Bacillus phages use a communication system, termed “arbitrium,” to coordinate lysis-lysogeny decisions. Arbitrium communication is mediated by the production and secretion of a hexapeptide (AimP) during lytic cycle. Once internalized, AimP reduces the expression of the negative regulator of lysogeny, AimX, by binding to the transcription factor, AimR, promoting lysogeny. We have elucidated the crystal structures of AimR from the Bacillus subtilis SPbeta phage in its apo form, bound to its DNA operator and in complex with AimP.

To establish the molecular basis of this novel mechanism of phage communication we produced crystals of AimR in its apo form that diffracted to 2.7Å and belong to space group P21 with eight monomers in the asymmetric unit. The overall structure of each monomer shows an N-terminal HTH DNA-binding domain (residues 1–59) directly connected (only 2 residues) to a C-terminal regulatory domain (residues 62–386) composed of 18 helices arranged in a two-layered right-handed superhelix. The HTH motif includes 4 helices (helix α1–α4), and the predicted DNA recognition helix α3 is solvent exposed, which is compatible with the active DNA-binding state proposed for the apo protein (Erez et al., 2017). Sequence analysis with TPRpred server (Zimmermann et al., 2018) only predicts the presence of four TPR, but the structure showed that the 18 α helices of C-terminal domain could be organized in 9 TPR-like motifs if helix α4 of the HTH domain was part of the first TPR. These 9 TPR-like motifs (TPR1–9), unlike other members of the RRNPP family, can be further divided in two subdomains, one N-terminal (TPRN-ter; residues 46–281), which would include helix α4 and encompasses six TPR motifs (TPR1–6), and the other C-terminal (TPRC-ter; residues 295–386), including the remaining three TPR motifs (TPR7–9). The eight monomers (A through H) of the asymmetric unit are arranged into four stable dimers characterized by an overall interface area of around 1,250 Å2. Structural comparison showed that each AimR monomer adopts a slightly different conformation, suggesting intrinsic plasticity for this protein. Protein domain motion analysis with Dyndom showed that this flexibility is due to the different relative disposition of two almost rigid portions, the first one including the HTH domain and the TPRN-ter, and the second one corresponding to the TPRC-ter with a bending region (281–285) placed in the TPR connector that would work as structural hinge. Interactions at the two ends of the TPR superhelix mediate AimR dimerization. The constant region of dimerization is nucleated by the interaction of the C-terminal α22 helices in TPR9, generating a helix bundle where also participate helices α20 from TPR8 that form a four-helix bundle. Although these two TPRs are involved in all the AimR apo dimer interactions, the specific contact changes among dimers, indicating that this region works through a slipping interface of contact.

>MELIRIAMKKDLENDNSLMNKWATVAGLKNPNPLYDFLNHDGKTFNEFSSIVNIVKSQYPDREYELMKDYCLNLDVKTKAARSALEYADANMFFEIEDVLIDSMISCSNMKSKEYGKVYKIHRELSNSVITEFEAVKRLGKLNIKTPEMNSFSRLLLLYHYLSTGNFSPMAQLIKQIDLSEISENMYIRNTYQTRVHVLMSNIKLNENSLEECREYSKKALESTNILRFQVFSYLTIGNSLLFSNYELAQENFLKGLSISVQNENYNMIFQQALCFLNNVWRKENKWINFESDSIMDLQEQAHCFINFNENSKAKEVLDKLDLLVHNDNELAMHYYLKGRLEQNKACFYSSIEYFKKSNDKFLIRLPLLELQKMGENQKLLELLLL[8x]(2R,4R)-1-methyl-4-hydroxyl-pyrrolidine-2-carboxylic acid | C6 H11 N O3 | 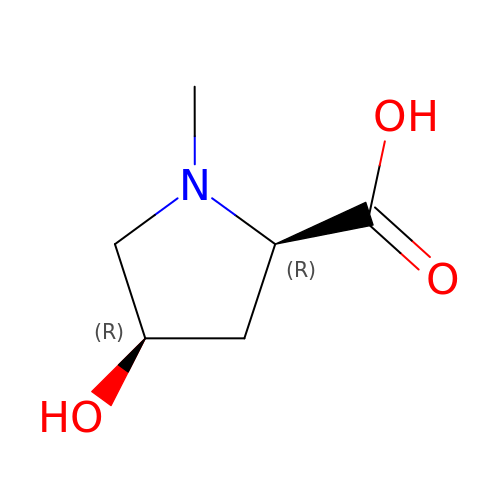FMIPNAUMSPFTHK-RFZPGFLSSA-N>[2x]SNADQTY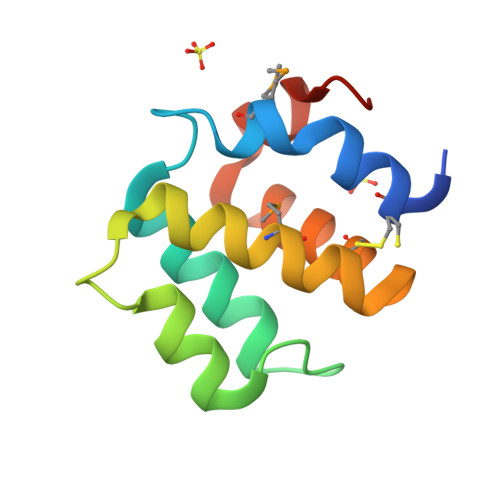CDRLVQDTPMLTGHGRLSEQQVDRIILQLNRYYPQILTNKEAEKFRNPKASLRVRLCDLMSHLQRSGERDCQEFYRALYIHAQPLHSRLPSRHAL> GSHMMHTLRLFTVLSLLLTSAFTLFPETETEVTPIQQLFLIKELKPGIARIGVIWDKNAANRDEVLPQLQRASAATGIK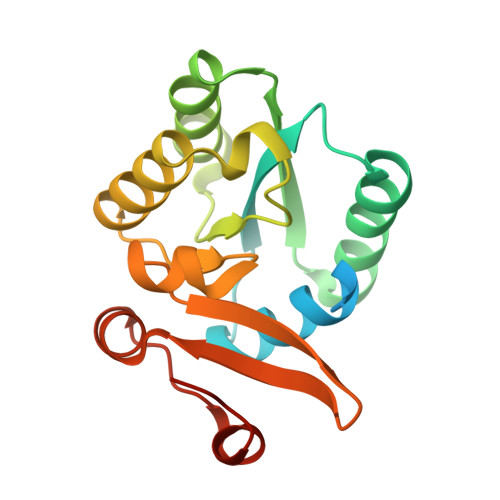VVVAEVASLQEVAPQFRTLLRDHQVEALWVLEESGLLGQAAARSFLIKNATQAGMPVFAPSETWLKEGACVTWRKDAEGIRLVVNKAVAEAMGITIPAKYQDRTAFLAMN3-fluoranyl-~{N}-methyl-5-[[1-oxidanylidene-6-[5-(trifluoromethyl)-1~{H}-pyrazol-4-yl]isoquinolin-2-yl]methyl]benzamide 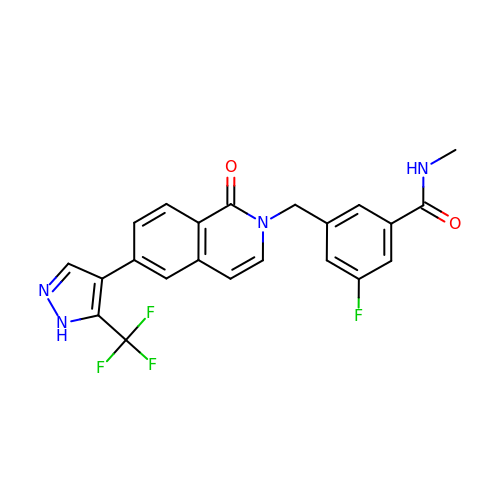| C22 H16 F4 N4 O2 | OCMZUTUUYBFIFC-UHFFFAOYSA-N>MSLTSEDFLIKSKGYLDIQTGEIIKADLLIRNGKIAEIGKINTKDATVISIPDLILIPGLMDSHVHIVGNDSKGEESIADSSHM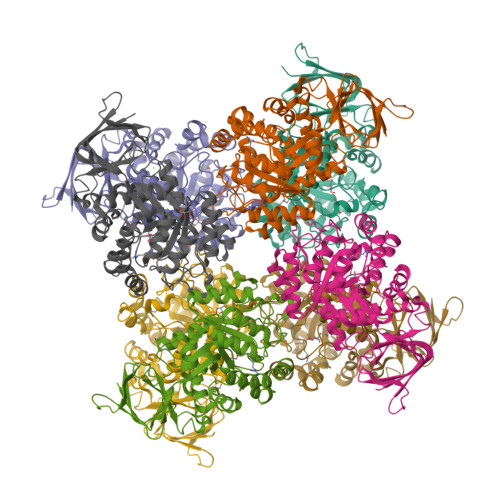GTVWGVVNAEKTLMAGFTTVRNVGAANYADVSVRDAIERGVINGPTMLVSGPALGITGGHCDHNLLPPEFNYSSEGVVDSPWEARKMVRKNRKYGADLIKFCATGGVMSRNTDVNAKQFTLEEMKAIVDEAHNHGMKVAAHAHGLIGIKAAIKAGVDSVEHASFIDDETIDMAIKNNTVLSMDIFVSDYILGEGAKAGIREESLNKERLVGKKQRENFMNAHRRGAIITFGTDAGIFDHGDNAKQFAYMVEWGMTPLEAIQASTIKTATLFGIENIGQIKEGFDADIVGVIENPLANIRTLEEVAFVMKEGKVYKREGHHHHHH[8x]> MASKAVILAGGLGTRLSEETIVKPKPMVEIGGKPILWHIMKMYSVHGIKDFIICCGYKGYVIKEYFANYFLHMSDVTFHMAENRMEVHHKRVEPWNVTLVDTGDSSMTGGRLKRVAEYVKDDEAFLFTYGDGVADLDIKAT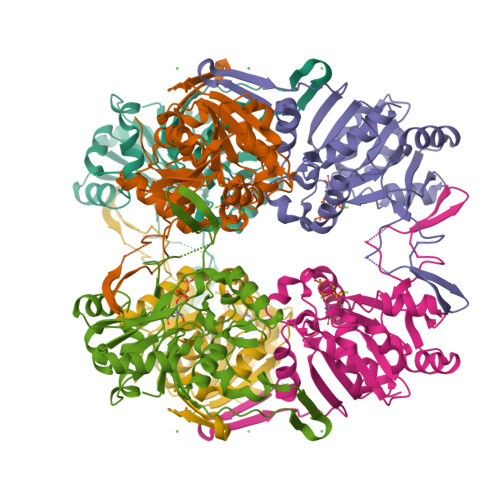IDFHKAHGKKATLTATFPPGRFGALDIQAGQVRSFQEKPKGDGAMINGGFFVLNPSVIDLIDNDATTWEQEPLMTLAQQGELMAFEHPGFWQPMDTLRDKVYLEGLWEKGKAPWKTWE> GSSTRDYEIQR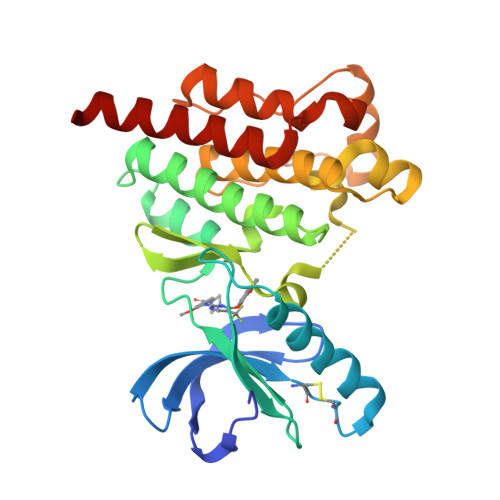ERIELGRCIGEGQFGDVHQGIYMSPENPALAVAIKTCKNCTSDSVREKFLQEALTMRQFDHPHIVKLIGVITENPVWIIMELCTLGELRSFLQVRKYSLDLASLILYAYQLSTALAYLESKRFVHRDIAARNVLVSSNDCVKLGDFGLSRYMEDSTYYKASKGKLPIKWMAPESINFRRFTSASDVWMFGVCMWEILMHGVKPFQGVKNNDVIGRIENGERLPMPPNCPPTLYSLMTKCWAYDPSRRPRFTELKAQLSTILEEEKAQQEE>[14x]TTTVGITLKDAVIMATERRVTMENFIMHKNGKKLFQIDTYTGMTIAG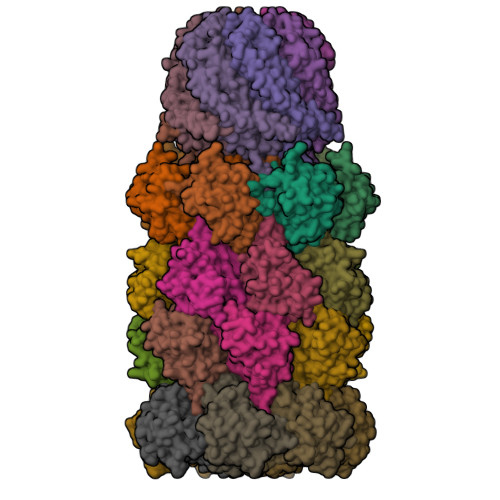LVGDAQVLVRYMKAELELYRLQRRVNMPIEAVATLLSNMLNQVKYMPYMVQLLVGGIDTAPHVFSIDAAGGSVEDIYASTGSGSPFVYGVLESQYSEKMTVDEGVDLVIRAISAAKQRDSASGGMIDVAVITRKDGYVQLPTDQIESRIRKLGLIL;>AYDRAITVFSPDGRLFQVEYAREAVKKGSTALGMKFANGVLLISDKKVRSRLIEQNSIEKIQLIDDYVAAVTSGLVADARVLVDFARISAQQEKVTYGSLVNIENLVKRVADQMQQYTQYGGVRPYGVSLIFAGIDQIGPRLFDCDPAGTINEYKATAIGSGKDAVVSFLEREYKENLPEKEAVTLGIKALKSSLEEGEELKAPEIASITVGNKYRIYDQEEVKKFL[7x];>[7x]KRAALIQNLRDSYTETSSFAVIEEWAAGTLQEIEGIAKAAVEAHGTIRNSTYGRAQAEKSPEQLLGVLQRYQDLCHNVYCQAETIRTVIAIRIPEHKEADNLGVAVQHAVLKVIDELEIKTLGSGEKSGSGGAPTPIGMYALREYLSARSTVEDKLLGSVDAESGKTKGGSQSPSLLLELRQIDADFMLKVELATTHLSTMVRAVINAYLLNWKKLIQPRGGHLDVLYR;>YDRAITVFSPDGRLFQVEYAREAVKKGSTALGMKFANGVLLISDKKVRSRLIEQNSIEAIQLIDDYVAAVTSGLVADARVLVDFARISAQQEKVTYGSLVNIENLVKRVADQMQQYTQYGGVRPYGVSLIFAGIDQIGPRLFDCDPAGTINEYKATAIGSGKDAVVSFLEREYKENLPEKEAVTLGIKALKSSLEEGEELKAPEIASITVGNKYRIYDQEEVKKFL[7x]> MEGERKNNNKRWYFTREQLENSPSRRFGVDPDKELSYRQQAANLLQDMGQRLNVSQLTINTAIVYMHRFYMIQSFTQFPGNSVAPAALFLAAKVEEQPKKLEHVIKVAHTCLHPQESLPDTRSEAYLQQVQDLVILESIILQTL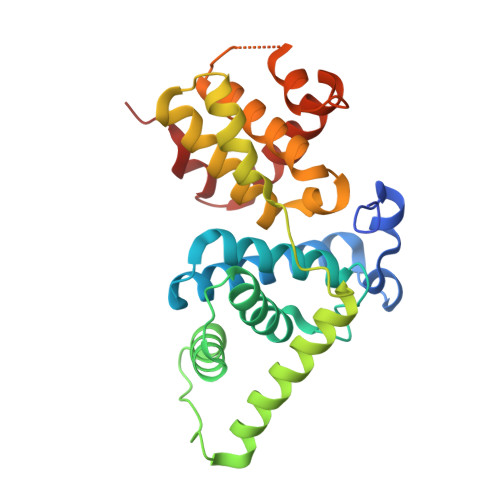GFELTIDHPHTHVVKCTQLVRASKDLAQTSYFMATNSLHLTTFSLQYTPPVVACVCIHLACKWSNWEIPVSTDGKHWWEYVDATVTLELLDELTHELLQILEKTPNRLKRIWNWR>SDPSTGLPNKLFAFIGKTTASTSYVEKNLLSSTTGAAMVGLPSGGNLLQAQYFVTPEQFGAIGDGVTDDTQAILKTITFANTNNIQVRADKNYRFTSSIAMSGVRWYGGTFTGNGGTMISTVSCWMENVRFEKCYVKMLGGDCRFYRNIFSNATSTAAFLMQAMTSEGTLDFSYNEMYGCKYAILQQGTGEVMTYGRYSNNYIHDIKGDAIELNVVQKHYTEGLIIENNHIANVDASGQGANWGIGIGVAGSGPYGVDVPDSQYVRNFSIVGNRVYNCRQCLHVEMGKNFTIRDNEVYPNTAVSTGTGLTTCGVALYGCQDFEVDGLTGYLLNDPSVSTRMVFIDWGVNNGRYAGPPINFTIKNLDIPESSIEIATSGSDAWENSTIVSNINCNVFKWRGLPSSSTFNNIRCRSIDFIGQHGSGEGSGGGFYTRSQFTYMKWVGCTALSGDETTVSFAKIYTDRC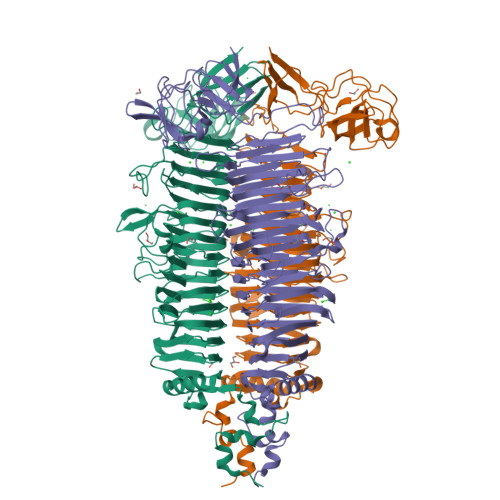DQVGNNFGVPTAVDGTGHRGPVLTTISEQYFTAYDEFPGGREFPTGTVIHCASGKKHVVTVGGAFFSDNEKIKATVTGQTYLQSNALNWASNGYAKAAGTKIVIPGAGANGGDLVTTIARATYVTNSLYTIDIADPIVTPTAENTQIKALNPVTFVTVNNA[3x]>GPLGSEVYKGDGYKVWKLEPSLGDPLELGRKTKT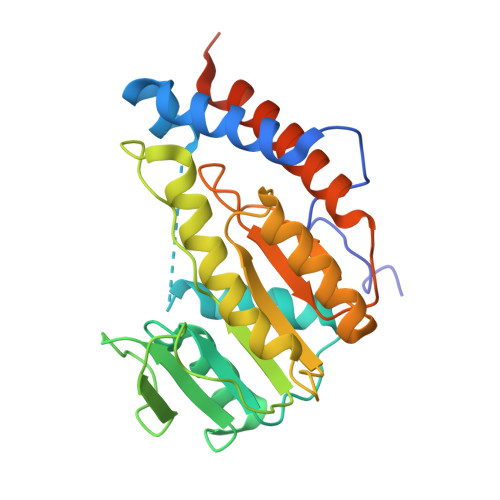EMNAMTHDEFDRMKYRGVVAEVYSGDKPSKGYDKLRVLLDLMDRPRLGTTVDLCAGRGGWSELVKDLEGPKGITAVSLWERGKEEWMADPAIHRINANVKHLRPWQVDTLLFDGGEAFKRDQNLRKEENFNDSLLDAVDAWMMQPVPPRNFVIKIQVPYTQKAIALLEKWQVKTGKGRLVRLAGDRLSNTVMYFLSVRLETQIRGRVTTFVRELAERRKDRSLTADPSLQYERVEPQWTEEAR[2x]> QEGDAAKGEKEFNKCKACHMVQAPDGTDIVKGGKTGPNLYGVVGRKIASVEGFKYGDGILEVAEKNPDMVWSEADLIEYVTDPKPWLVEKTGDSAAKTKMTFKLGKNQADVVAFLAQHSPDAGAEAAPAEGA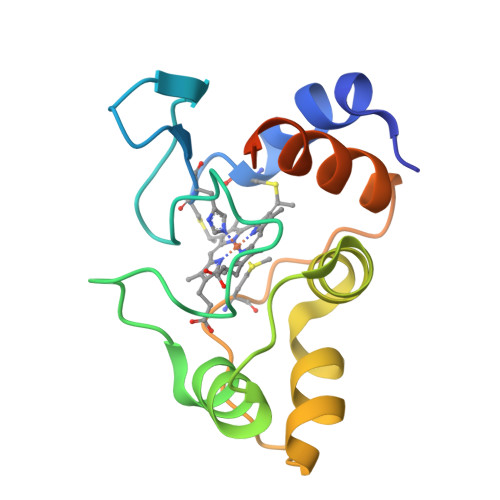AN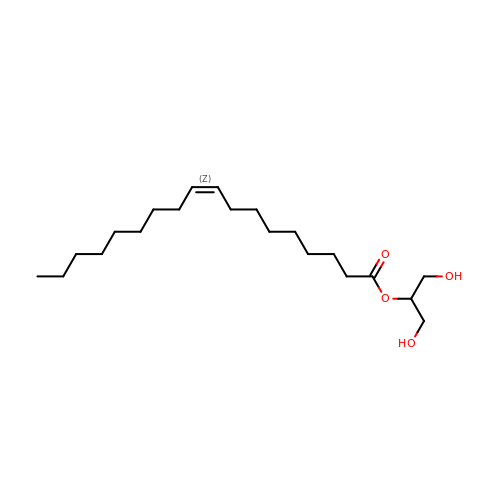1,3-dihydroxypropan-2-yl (9Z)-octadec-9-enoate | C21 H40 O4 | UPWGQKDVAURUGE-KTKRTIGZSA-N>[4x]AEAPATRKDC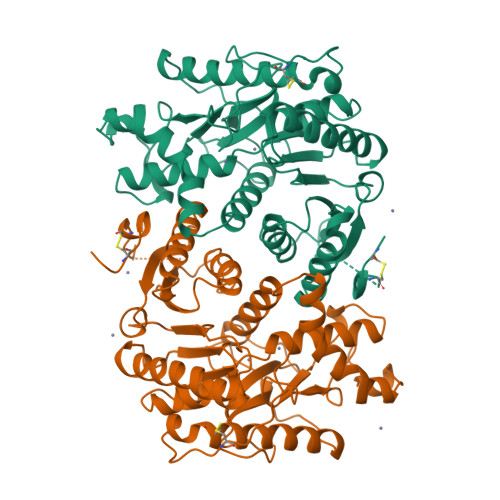FGVFCTTYDLKAEDKTKSWKKLVNIAVSGAAGMISNHLLFKLASGEVFGQDQPIALKLLGSERSFQALEGVAMELEDSLYPLLREVSIGIDPYEVFEDVDWALLIGAKPRGPGMERAALLDINGQIFADQGKALNAVASKNVKVLVVGNPCNTNALICLKNAPDIPAKNFHALTRLDENRAKCQLALKAGVFYDKVSNVTIWGNHSTTQVPDFLNAKIDGRPVKEVIKRTKWLEEEFTITVQKRGGALIQKWGRSSAASTAVSIADAIKSLVTPTPEGDWFSTGVYTTGNPYGIAEDIVFSMPCRSKGDGDYELATDVSNDDFLWERIKKSEAELLAEKKCVAHLTGEGNAYCDVPEDTMLPGEV>SNAMHTALINHIRKFIFLTDEDAGTLSAFFQLKKVRKKETLLKTGEICRINYFVVKGCLRLFFIDEKGIEQTTQFAIENWWLSDYMAFQKQQPADFYIQSVENCELLSITYTEQENLFERIPALERYFRLVYQKSFAAAQLRSKFQHMYSKEEQYHNFS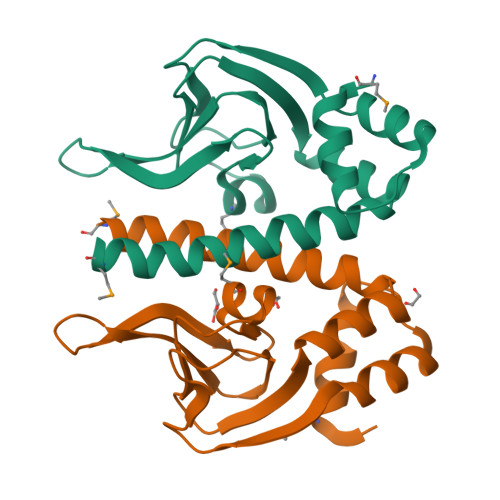SRFPEFIQRVPQYLLASYLGFTPEYLSEIRKKYIS[2x]> MSLETDDQYYRAIKKIKEAAEASNRAYL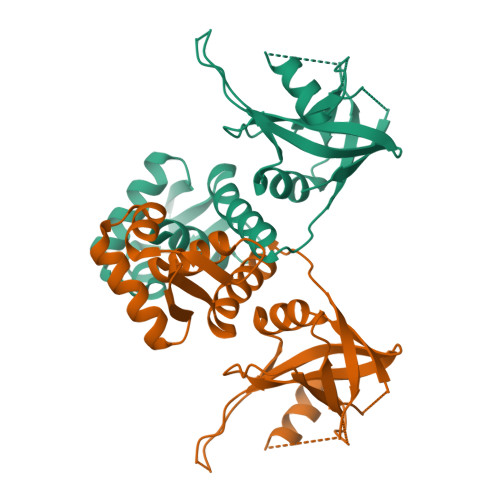TSSKLADMLGISQQSASRIIIDLEKNGYITRTVTKRGQILNITEKGLDVLYTEFADLSRILAIKNNVVITGTVTSGMGEGRYYVARKQYIIQFQEKLGIIPYLGTLNIKVDQASLPELRKIRGFRGIHIEGFKTEDRTFGSVKAFPAKIQNIPCFVIMPERTVYTDVIEIISDKYLREEINLHDGDRVSVEVYTEGHHHHHH>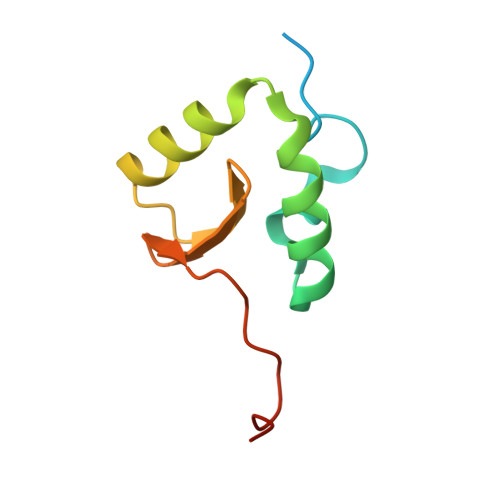 MSVLTVPRQTPRQRLPVLPCHVGDPDLWFADTPAGLEVAKTLCVSCPIRRQCLAAALQRAEPWGVWGGEIFDQGSIVSHKRPRGRPRKDAVA>RPSWSPTQASGQTVLPF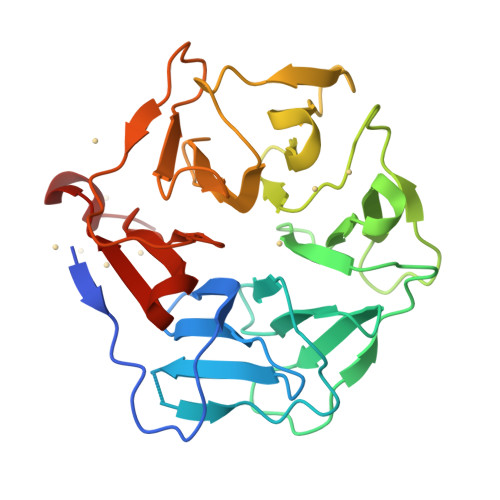TGIDFRLSPSGVAVDSAGNVYVTSEGMYGRVVKLATGSTGTTVLPFNGLYQPQGLAVDGAGTVYVTDFNNRVVTLAAGSNNQTVLPFDGLNYPEGLAVDTQGAVYVADRGNNRVVKLAAGSKTQTVLPFTGLNDPDGVAVDNSGNVYVTDTDNNRVVKLEAESNNQVVLPFTDITAPWGIAVDEAGTVYVTEHNTNQVVKLLAGSTTSTVLPFTGLNTPLAVAVDSDRTVYVADRGNDRVVKLTSLEHHHHHH[2x]> EPPLVFEPVTLESLRQEKGFQKVGKKQIKELDTLRKKHAKERTSVQKTQNAAIDKLIKGKSKDDIRNDANIKNSINDQTKQWTDMIARHRKEEWDMLRQHVQDSQDAMKALMLTVQAAQIKQLEDRHARDIKDLNAKQAKMSADTAKEVQNDKTLKTKNEKDRRLREKRQNNVKRFMEEKKQIGVKQGRAMEKLKLAHSKQIEEFSTDVQKLMDMYKIEEEAYKTQGKTEFYA

At the inner surface of fly photoreceptor rhabdomeric membranes, the master scaffold protein INAD (encoded by inaD for inactivation no after potential D and contains 5 PDZ domains arranged in tandem) forms stoichiometric multi-molecular complexes with phospholipase Cβ (NORPA), Ca2+-permeable transient receptor potential (TRP) channel and eye-specific protein kinase C (eye-PKC). In this study, we show that the PDZ45 tandem of INAD functions as a supramodule binding to the entire C-terminal coiled-coil domain and PDZ-binding motif of NORPA (CC-PBM) with an unexpectedly high affinity. Our biochemical and structural studies demonstrate that INADL PDZ89 forms a supramodule and binds to the entire C-terminal coiled-coil domain of PLCβ4 in a manner that is strikingly similar to that of the INAD–NORPA complex. The striking similarity between the PDZ scaffold and PLCβ interactions at the molecular level might point to an evolutionarily conserved molecular adaption in PLCβ signaling in the animal kingdom.

Confronted by this disappointing result, we decided to take a step back and tried to solve the NORPA CC-PBM structure alone first, hoping to be able to get some clues that might lead us to a way to obtain PDZ45–NORPA CC-PBM complex crystals (the structure of INAD PDZ45 was solved in our earlier study). Using lysine reductive-methylated protein, we were able to solve the structure of NORPA CC-PBM at the resolution of 3.0 Å. Like the coiled-coil structure of mammalian PLCβ3, NORPA CC folds into an elongated three helix bundle structure with an N-terminal short helix coupling to the middle region of the helix bundle. The C-terminal 16 residues (aa 1080–1095) that include the PBM is disordered and invisible in the structure. The packing surface of NORPA CC-PBM crystals involves an extensive surface composed of α1–α4. We reasoned that this packing surface might overlap with the INAD PDZ45 binding surface, and therefore prevented the same surface from being used for crystal packing in the PDZ45–NORPA CC-PBM complex. We noted that the solvent-exposed face of the α2 helix is lined with eight Lys residues, which are all evolutionarily conserved and required for the membrane binding of NORPA CC (and see below for more details).> MTTAARRPAPTTAGAGWDAGVGALVNPSRR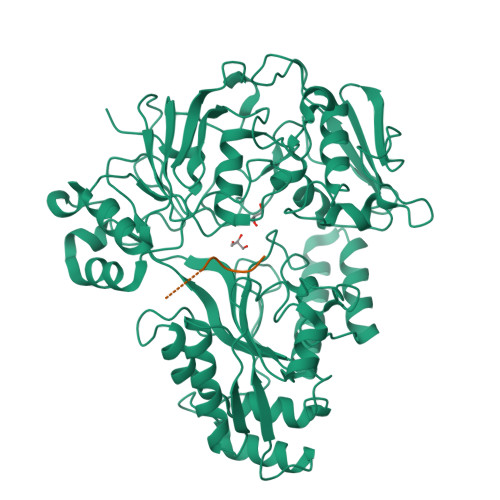RGGTLRLVSSADVDSLDPARTYYVWVWLLQRLLNRTLMAYPTDPGPAGLVPAPDLAEGPGEVSDGGRTWTYRLRRGLRYDDGTPITSDDVRHAVQRVFAQDVLPGGPTYLIPLLDDPERPYPGPYRTDEPLRSVLTPDEHTIVFRLTRPFSDFDHLMAQPCAAPVPRRSDTGADYGRDPRSSGPYRVARHEPDTLLHLERNPHWDRATDPIRPALPDRVELTIGLDVDVLDARLIAGEFDINLEGRGLQHAAQRRATADEVLRSHTDNPRTSFLHFVAMQPHIPPFDNVHVRRAVQYAADKILLQDARGGPVNGGDLTTALFPPTLPAHQDLDLYPTGPDLRGDLDAARAELAAAGLPDGFRAVIGTQRGKFRLVADAVVESLARVGIELTVKELDVATYFSLGAGHPETVREHGLGLLVTDWGADFPTEYGFLAPLVDGRQIKRNGGNWNLPELDDPEVNALIDETLHTTDPAARAELWRAVERRVMEHAVLLPLVHDKTLHFRNPWVTNVYVHPAFGLYDIQAMGLAEED;> RPPGFSPFR The multi-domain nonstructural protein 3 (nsp3) is the largest protein encoded by the known coronavirus genome and serves as a central component of the viral replication and transcription machinery. Nsp3 can be divided into three parts, including a large N-terminal cytosolic region (~ 157 kDa in SARS-CoV-2 with ten distinct domains) followed by a transmembrane region (~ 20 kDa with three domains) and a C-terminal cytosolic region (~ 41 kDa with two domains). On the other hand, little is known about structures of the transmembrane and C-terminal regions of nsp3 or their exact function in the viral replication cycle. This part of nsp3 consists of two transmembrane domains (TM1 and TM2) separated by a luminal ectodomain (3Ecto) and two Y domains (referred to as Y1 and CoV-Y) in the C terminus. Previous studies demonstrated that the highly-conserved C-terminal region of nsp3 is essential for subcellular membrane rearrangement, yet the underlying mechanisms remain elusive.

In an effort to understand the role of the nsp3 Y domains in the coronavirus replication cycle, we have determined the crystal structure of the 286-residue CoV-Y domain of the SARS-CoV-2 nsp3, the first complete CoV-Y domain structure for any known coronavirus. As a result, a shorter construct (residues 1660–1945) was designed and used for subsequent NMR and X-ray crystallography studies. The structure was determined and refined at a resolution of 2.4 Å by multiple-wavelength anomalous dispersion using data collected from a selenomethionine-substituted crystal. The completed electron density map allowed unambiguous tracing of most of the protein except the five N-terminal residues (residues 1660–1664). The CoV-Y domain of SARS-CoV-2 nsp3 has a twisted structure resembling a letter V with linear dimensions of approximately 60 Å × 50 Å × 32 Å. The 2.4 Å-resolution structure reveals that CoV-Y possesses a previously uncharacterized V-shaped fold consisting of three distinct subdomains named Y2, Y3 and Y4. The N-terminal Y2 subdomain (residues 1665–1763) is dominated by six β strands (S21–S26) arranged into two nearly orthogonal β sheets (S21↑S26↑S25↑ on one sheet and S22↑S23↓S24↑ on the other) to form a β sandwich-like structure packed across a hydrophobic core. The middle Y3 subdomain (residues 1764–1847) adopts a compact α helical fold composed of a three-helix bundle (H31–H33) packing against the 4th helix (H34) with an axial tilt of ~ 60°. The C-terminal Y4 subdomain (residues 1848–1945) consists of a α/β fold with two three-stranded β sheets (S41↑S45↑S44↑ and S42↓S43↓S46↑) in the center flanked by three α helices (H42–H44) and a 310 helix (H41). Y4 packs tightly against Y3 and the Y3–Y4 interface is dominated by hydrophobic interactions between H34 of Y3 and H44 and S45 of Y4.

> GKRPINPTDQSSYIVDSVTVKNGSIHLYFDKAGQKTYERHSLSHFVNLDNLRANNTKGSLPINVIVFDGKSKCEESSAKSASVYYSQLMCQPILLLDQALVSDVGDSAEVAVKMFDAYVNTFSSTFNVPMEKLKTLVATAEAELAKNVSLDNVLSTFISAARQGFVDSDVETKDVVECLKLSHQSDIEVTGDSCNNYMLTYNKVENMTPRDLGACIDCSARHINAQVAKSHNIALIWNVKDFMSLSEQLRKQIRSAAKKNNLPFKLTCATTRQVVNVVTTKIALKGG Calbindin-D28K is a major calcium-buffering cytoplasmic protein that is expressed at particularly high levels in the central nervous system (CNS) and absorptive epithelium (gut and kidney; Schmidt, 2012). Not only does calbindin-D28K act as a buffer for calcium ions, but it has also been shown to interact with multiple protein targets to modulate their function or catalytic activity. Calbindin-D28K belongs to a superfamily of calcium-binding proteins that includes calmodulin and troponin C. All of these proteins have a high α-helical content and share EF-hand structures that constitute the calcium-binding domains. Calbindin-D28K has a primary structure of 261 amino acids (molecular mass of ∼30 kDa) and is encoded by the CALB1 gene.

Here, we report the first X-ray structure of calbindin-D28K, allowing the first detailed high-resolution analysis of its calcium-binding properties. Five amino-acid residues, a backbone interaction and a water molecule complete the coordination of calcium in the EF1, EF4 and EF5 motifs. In contrast, the EF3 motif utilizes an interaction at Glu119 (position 9) instead of a water molecule to complete the coordination of calcium. At position 12 all four calcium-binding loops possess a conserved glutamate side chain that acts as a bidentate coordinating residue. Calcium binding at the N-terminal EF-hand (EF1) motif (where the electron density is more disordered) appears to be more flexible that in the other calcium-binding loops. Calcium SAD at long wavelength demonstrated that the N-terminal EF-hands are particularly flexible and possesses two calcium-binding conformations. Nevertheless, the N-terminal flexibility still manifests as structural disorder, with higher temperature-factor values in this region. It was not possible to build the two conformations into the electron density, and only one calcium-binding site is visible in the final structure. Here, we demonstrate that Asp24 and Asp26 are involved in calcium binding. Compared with the existing NMR model of calbindin-D28K, the X-ray structure is less compact, with the intramolecular distances increased by several ångströms across the molecule.

> GPHMAESHLQSSLITASQFFEIWLHFDADGSGYLEGKELQNLIQELQQARKKAGLELSPEMKTFVDQYGQRDDGKIGIVELAHVLPTEENFLLLFRCQQLKSCEEFMKTWRKYDTDHSGFIETEELKNFLKDLLEKANKTVDDTKLAEYTDLMLKLFDSNNDGKLELTEMARLLPVQENFLLKFQGIKMCGKEFNKAFELYDQDGNGYIDENELDALLKDLCEKNKQDLDINNITTYKKNIMALSDGGKLYRTDLALILCAGDN>MSVPKKRNHGKLPPSTKDVDDPSLKYTKAAPKCEQVAEHWLLQPLPEPESRYSFWVTIVTLLAFAARFYKIWYPKEVVFDEVHFGKFASYYLERSYFFDVHPPFAKMMIAFIGWLCGYDGSFKFDEIGYSYETHPAPYIAYRSFNAILGTLTVPIMFNTLKELNFRAITCAFASLLVAIDTAHVTETRLILLDAILIISIAATMYCYVRFYKCQLRQPFTWSWYIWLHATGLSLSFVISTKYVGVMTYSAIGFAAVVNLWQLLDIKAGLSLRQFMRHFSKRLNGLVLIPFVIYLFWFWVHFTVLNTSGPGDAFMSAEFQETLKDSPLSVDSKTVNYFDIITIKHQDTDAFLHSHLARYPQRYEDGRISSAGQQVTGYTHPDFNNQWE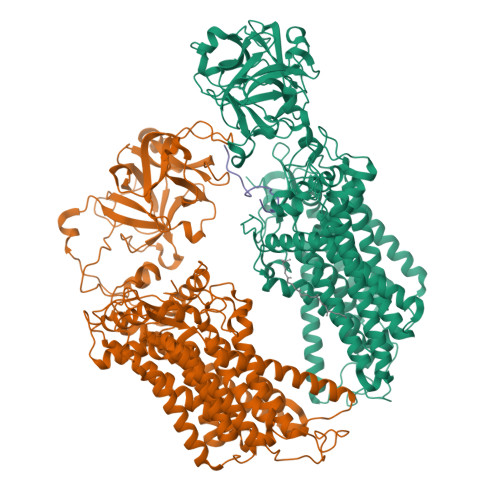VLPPHGSDVGKGQAVLLNQHIRLRHVATDTYLLAHDVASPFYPTNEEITTVTLEEGDGELYPETLFAFQPLKKSDEGHVLKSKTVSFRLFHVDTSVALWTHNDELLPDWGFQQQEINGNKKVIDPSNNWVVDEIVNLDEVRKVYIPKVVKPLPFLKKWIETQKSMFEHNNKLSSEHPFASEPYSWPGSLSGVSFWTNGDEKKQIYFIGNIIGWWFQVISLAVFVGIIVADLITRHRGYYALNKMTREKLYGPLMFFFVSWCCHYFPFFLMARQKFLHHYLPAHLIACLFSGALWEVIFSDCKSLDLEKDEDISGASYERNPKVYVKPYTVFLVCVSCAVAWFFVYFSPLVYGDVSLSPSEVVSREWFDIELNFSK[2x];> TSTNATSSSCATPSLK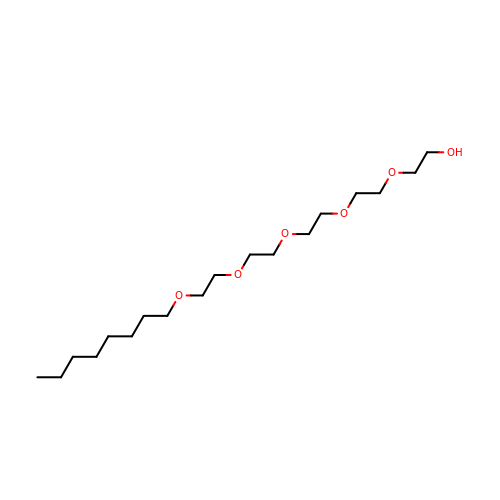3,6,9,12,15-PENTAOXATRICOSAN-1-OL | C18 H38 O6 | MJELOWOAIAAUJT-UHFFFAOYSA-N>SMTDQAFVTLTTNDAYAKGALVLGSSLKQHRTTRRLVVLATPQV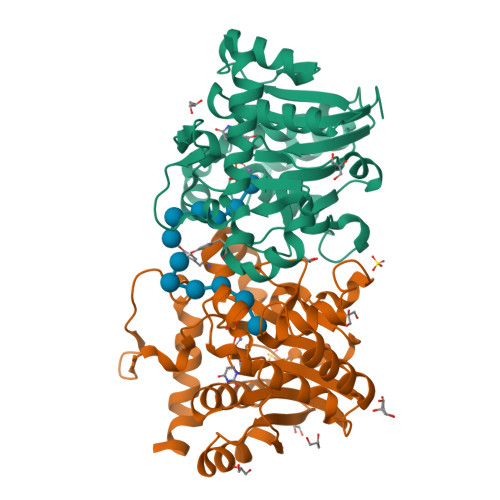SDSMRKVLETVFDEVIMVDVLDSGDSAHLTLMKRPELGVTLTKLHCWSLTQYSKCVFMDADTLVLANIDDLFDREELSAAPDPGWPDCFNSGVFVYQPSVETYNQLLHLASEQGSFDGGDQGILNTFFSSWATTDIRKHLPFIYNLSSISIYSYLPAFKVFGASAKVVHFLGRVKPWNYTYDPKTKSVKSEAHDPNMTHPEFLILWWNIFTTNVLPLLQ[2x]>[3x]AERSLLTGE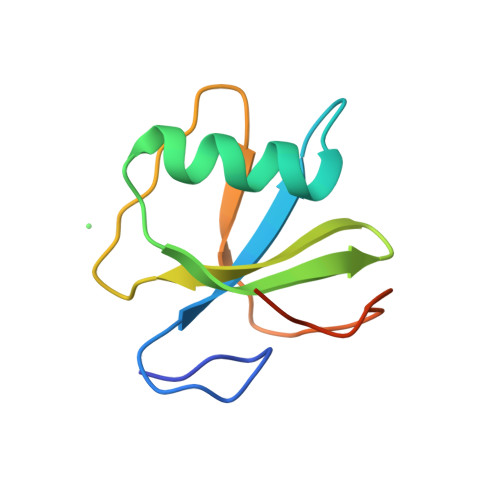EGWRTYKATGPRLSLPRLVALLKGQGLEVGAVAEAEGGFYVDLRPEARPEVAGLRLEPARRVEGLLEIPSRTRRPARA> MNTINIAKNDFSDIELAAIPFNTLADHYGERLAREQLALEHESYEMGEARFRKMFERQLKAGEVADNAAAKPLITTLLPKMIARINDWFEEVKAKRGKRPTAFQFLQEIKPEAVAYITIKTTLACLTSADNTTVQAVASAIGRAIEDEARFGRIRDLEAKHFKKNVEEQLNKRVGHVYKKAFMQVVEADMLSKGLLGGEAWSSWHKEDSIHVGVRCIEMLIESTGMVSLHRQNAGVVGQDSETIELAPEYAEAIATRAGALAGISPMFQPCVVPPKPWTGITGGGYWANGRRPLALVRTHSKKALMRYEDVYMPEVYKAINIAQNTAWKINKKVLAVANVITKWKHCPVEDIPAIEREELPMKPEDIDMNPEALTAWKRAAAAVYRKDKARKSRRISLEFMLEQANKFANHKAIWFPYNMDWRGRVYAVSMFNPQGNDMTKGLLTLAKGKPIGKEGYYWLKIHGANCAGVDKVPFPERIKFIEENHENIMACAKSPLENTWWAEQDSPFCFLAFCFEYAGVQHHGLSYNCSLPLAFDGSCSGIQHFSAMLRDEVGGRAVNLLPSETVQDIYGIVAKKVNEILQADAINGTDNEVVTVTDENTGEISEKVKLGTKALAGQWLAYGVTRSVTKRSVMTLAYGSKEFGFRQQVLEDTIQPAIDSGKGLMFTQPNQAAGYMAKLIWESVSVTVVAAVEAMNWLKSAAKLLAAEVKDKKTGEILRKRCAVHWVTPDGFPVWQEYKKPIQTRLNLMFLGQFRLQPTINTNKDSEIDAHKQES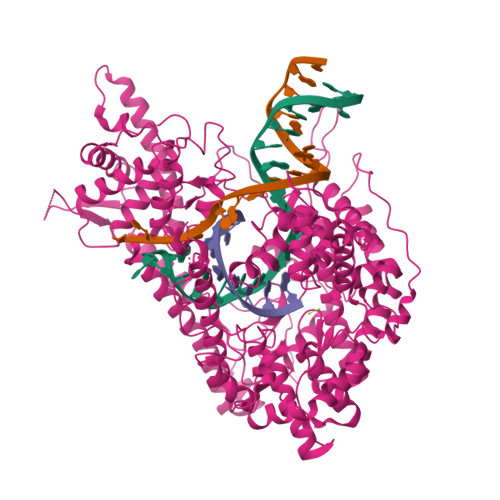GIAPNFVHSQDGSHLRKTVVWAHEKYGIESFALIHDSFGTIPADAANLFKAVRETMVDTYESCDVLADFYDQFADQLHESQLDKMPALPAKGNLNLRDILESDFAFA> MPRPSAGSHHNDKLHFKKGDTVIVLSGKHKGQTGKVLLALPRDQKVVVEGVNVITKNVKPSMTNPQGGQEQRELALHASKVALV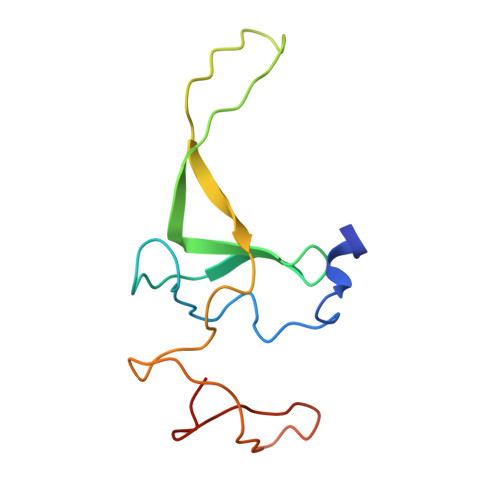DPETGKATRVRKQIVDGKKVRVAVASGKTID> FFAALL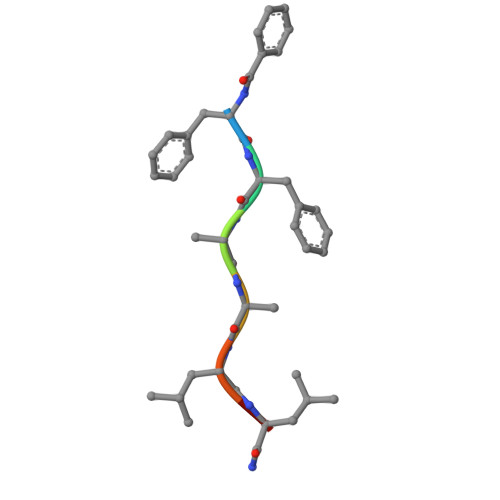X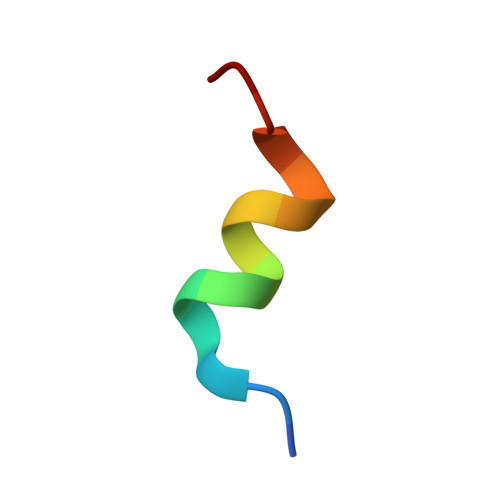> HVERLQIFQHLHPIV> MRAKIPSEEVAVKLNEWYKLIRAFEADQAEALKQEIEYDLEDMEENQDLLLYFSLMEFRHRIMLDKLMPVKDSDTKPPFSDMLNEIESNQQKLTGLLEYYFYYFRGMYEFKQKNFILAIDHYKHAEEKLEYVEDEIEKAEFLFKVAEVYYHIKQTYFSMNYASQALDIYTKYELYGRRRVQCEFIIAGNLTDVYHHEKALTHLCSALEHARQLEEAYMIAAAYYNVGHCKYSLGDYKEAEGYFKTAAAIFEEHNFQQAVQAVFSLTHIYCKE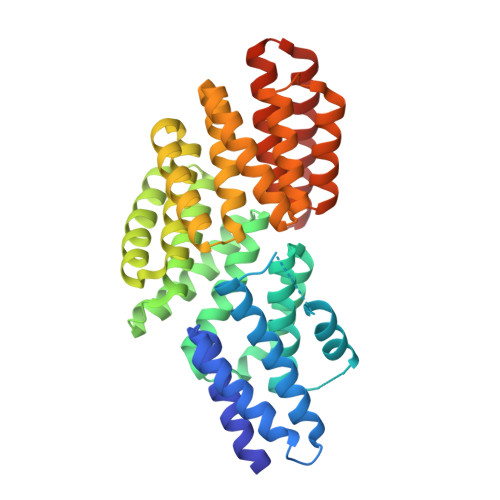GKYDKAVEAYDRGIKSAAEWEDDMYLTKFRLIHELYLGSGDLNVLTECFDLLESRQLLADAEDLLHDTAERFNQLEHYESAAFFYRRLMNIKKKLAEQRFQ>EFVFEWFGSNESGAEFGTNIPGVWGTDYIFPDPSAISTLIDKGMNFFRVQFMMERLLPDSMTGSYDEEYLANLTTVIKAVTDGGAHALVDPHNYGRYNGEIISSTSDFQTFWENLAGQYKDNDLVMFDTNNEYHDMDQDLVLNLNQAAINGIRAAGATSQYIFVEGNSWTGAWTWVDVNDNMKNLTDPEDKIVYEMHQYLDSDGSGTSETCVSETIGKERVTEATQWLKDNKKVGFIGAYAGGSND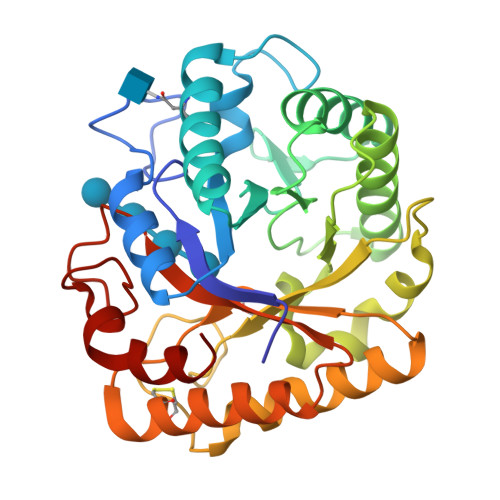VCRSAVSGMLEYMANNTDVWKGASWWAAGPWWGDYIFSLEPPDGTAYTGMLDILEAYL[2x]>[2x]GSHMASSHLAELVASAKAAISQASDVAALDNVRVEYLGKKGHLTLQMTTLRELPPEERPAAGAVINEAKEQVQQALNARKAELESAALNARLAAETIDVSLPGRRIENGGLHPVTRTIDRIESFFGELGFTVATGPEIEDDYHNFDALNIPGHHPARADHDTFWFDTTRLLRTQTSGVQIRTMKAQQPPIRIIAPGRVYRNDYDQTHTPMFHQMEGLIVDTNISFTNLKGTLHDFLRNFFEEDLQIRFRPSYFPFTEPSAEVDVMGKNGKWLEVLGCGMVHPNVLRNVGIDPEVYSGFAFGMGMERLTMLRYGVTDLRSFFENDLRFLKQFK;>MKFSELWLREWVNPAIDSDALANQITMAGLEVDGVEPVAGSFHGVVVGEVVECAQHPNADKLRVTKVNVGGDRLLDIVCGAPNCRQGLRVAVATIGAVLPGDFKIKAAKLRGEPSEGMLCSFSELGISDDHSGIIELPADAPIGTDIREYLKLDDNTIEISVTPNRADCLGIIGVARDVAVLNQLPLVQPEIVPVGATIDDTLPITVEAPEACPRYLGRVVKGINVKAPTPLWMKEKLRRCGIRSIDAVVDVTNYVLLELGQPMHAFDKDRIEGGIVVRMAKEGETLVLLDGTEAKLNADTLVIADHNKALAMGGIFGGEHSGVNDETQNVLLECAFFSPLSITGRARRHGLHTDASHRYERGVDPALQHKAMERATRLLIDICGGEAGPVIDITNEATLPKRATITLRRSKLDRLIGHHIADEQVTDILRRLGCEVTEGKDEW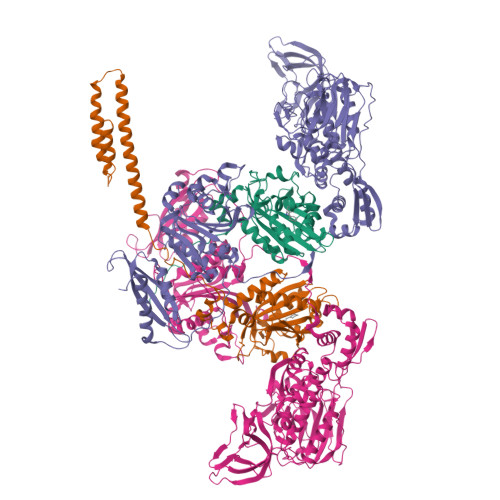QAVAPSWRFDMEIEEDLVEEVARVYGYNNIPDEPVQASLIMGTHREADLSLKRVKTLLNDKGYQEVITYSFVDPKVQQMIHPGVEALLLPSPISVEMSAMRLSLWTGLLATVVYNQNRQQNRVRIFESGLRFVPDTQAPLGIRQDLMLAGVICGNRYEEHWNLAKETVDFYDLKGDLESVLDLTGKLNEVEFRAEANPALHPGQSAAIYLKGERIGFVGVVHPELERKLDLNGRTLVFELEWNKLADRVVPQAREISRFPANRRDIAVVVAENVPAADILSECKKVGVNQVVGVNLFDVYRGKGVAEGYKSLAISLILQDTSRTLEEEEIAATVAKCVEALKERFQASLRD[2x]> MANMEARNVMSGTWGELWLDGNKVAEVKKFQAKMEFTKEDIIIAGQMGTDTKYMGYKGKGSITLYHVSSRMHKLIGEKIKRGSEPRFVAISKLNDPDSYGAERIAVK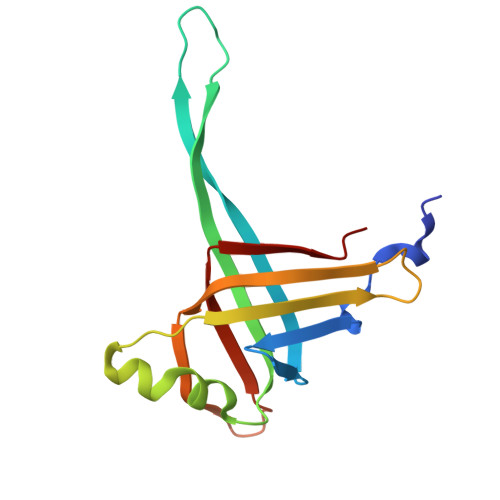NIAFDDLTLADWEVGVKGEIEAPFTFTEYDFLDII> AANAVANICQATNTQLYQLVEWAKHIPHFSSLPIEDQVLLLRAGWNELLIAAFSHRSVEVRDGIVLGAGITVHRNSAHQAGVGTIFDRVLTELVAKMRDMNMDRTELGSLRSIILFNPEVRGLKSGQEVELLREKVYAALEEYTRVTRPEEPGRFAKLLLRLPALRSIGLKCLEHLFFFRLIGDIP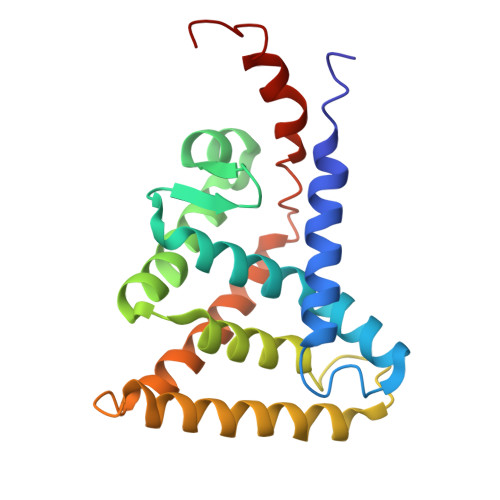IDTFLMDMLG N-(2-phenylethyl)acetamide | C10 H13 N O | 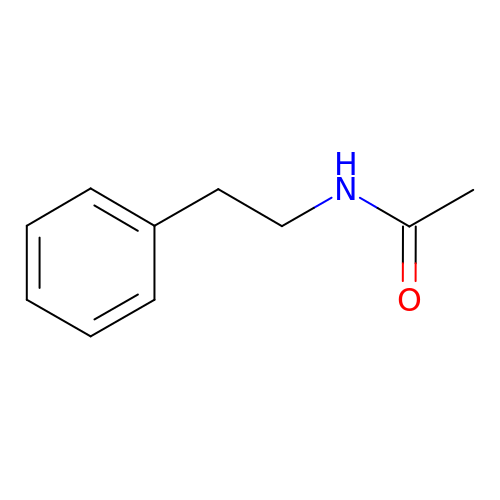MODKMHXGCGKTLE-UHFFFAOYSA-N>GSHMDQDSLSSSLKTCYKYLNQTSRSFAAVIQALDGEMRNAVCIFYLVLRALDTLEDDMTISVEKKVPLLHNFHSFLYQPDWRFMESKEKDRQVLEDFPTISLEFRNLAEKYQTVIADICRRMGIGMAEFLDKHVTSEQEWDKYCHYVAGLVGIGLSRLFSASEFEDPLVGEDTERANSMGLFLQKTNIIRDYLEDQQGGREFWPQEVWSRYVKKLGDFAKPENIDLAVQCLNELITNALHHIPDVITYL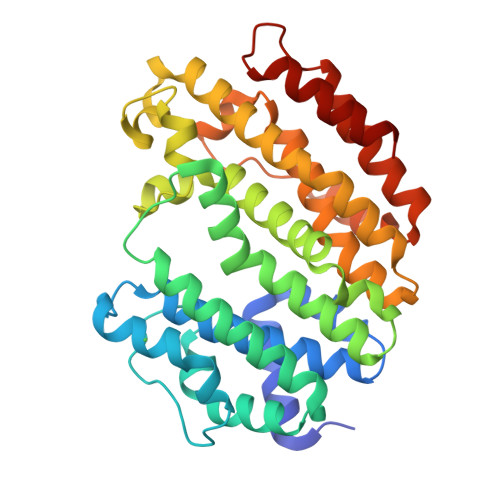SRLRNQSVFNFCAIPQVMAIATLAACYNNQQVFKGAVKIRKGQAVTLMMDATNMPAVKAIIYQYMEEIYHRIPDSDPSSSKTRQIISTIRTQN[2x]>SKIVKIIGREIIDSRGNPTVEAEVHLEGGFVGMAAAPSGASTGSREALELRDGDKSRFLGKGVTKAVAAVNGPIAQALIGKDAKDQAGIDKIMIDLDGTENKSKFGANAILAVSLANAKAAAAAKGMPLYEHIAELNGTPGKYSMPVPMMNIINGGEHADNNVDIQEFMIQPVGAKTVKEAIRMGSEVFHHLAKVLKAKGMNTAVGDEGGYAPNLGSNAEALAVIAEAVKAAGYELGKDITLAMDCAASEFYKDGKYVLAGEGNKAFTSEEFTHFLEELTKQYPIVSIEDGLDESDWDGFAYQTKVLGDKIQLVGDDLFVTNTKILKEGIEKGIANSILIKFNQIGSLTETLAAIKMAKDAGYTAVISHRSGETEDATIADLAVGTAAGQIKTGSMSRSDRVAKYNQLIRIEEALGEKAPYNGRKEIKGQA[4x];>ASPELASGK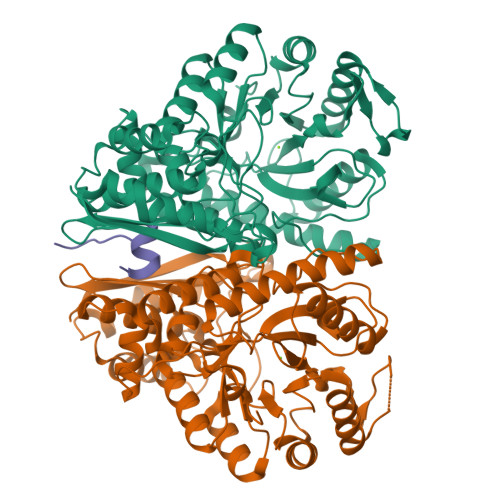VWIRYPIVR[2x]5-[(2S)-1-methylpyrrolidin-2-yl]pyridin-2-ol | C10 H14 N2 O | 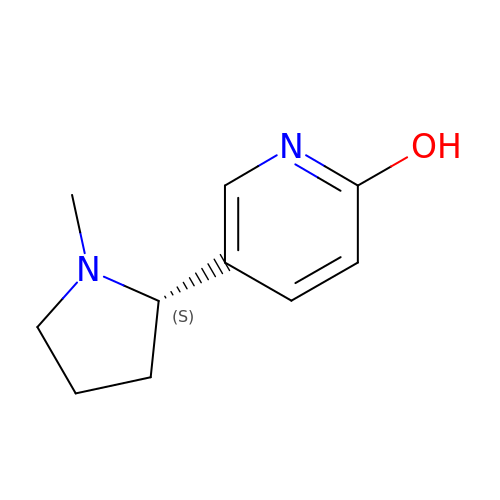ATRCOGLZUCICIV-VIFPVBQESA-N> MAGAIENARKEIKRISLEDHAESEYGAIYSVSGPVVIAENMIGCAMYELVKVGHDNLVGEVIRIDGDKATIQVYEETAGLTVGDPVLRTGKPLSVELGPGLMETIYDGIQRPLKAIKEESQSIYIPRGIDTPALDRTIKWQFTPGKFQVGDHISGGDIYGSVFENSLISSHKILLPPRSRGTITWIAPAGEYTLDEKILEVEFDGKKSDFTLYHTWPVRVPRPVTEKLSADYPLLTGQRVLDALFPCVQGGTTCIPGAFGCGKTVISQSLSKYSNSDAIIYVGCGERGNEMAEVLMEFPELYTEMSGTKEPIMKRTTLVANTSNMPVAAREASIYTGITLAEYFRDQGKNVSMIADSSSRWAEALREISGRLGEMPADQGFPAYLGAKLASFYERAGKAVALGSPDRTGSVSIVAAVSPAGGDFSDPVTTATLGITQVFWGLDKKLAQRKHFPSINTSVSYSKYTNVLNKFYDSNYPEFPVLRDRMKEILSNAEELEQVVQLVGKSALSDSDKITLDVATLIKEDFLQQNGYSTYDAFCPIWKTFDMMRAFISYHDEAQKA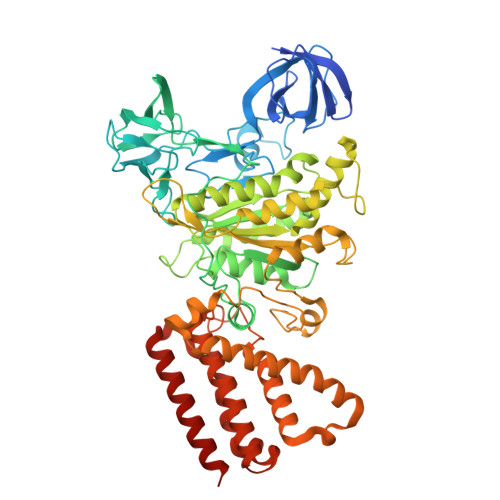VANGANWSKLADSTGDVKHAVSSSKFFEPSRGEKEVHGEFEKLLSTMQERFAESTD>MPQSKSRKIAILGYRSVGKSSLTIQFVEGQFVDSNDPTIENTFTKLITVNGQEYHLQLVDTAGQDEYSIFPQTYSIDINGYILVYSVTSIKSFEVIKVIHGKLLDMVGKVQIPIMLVGNKKDLHMERVIS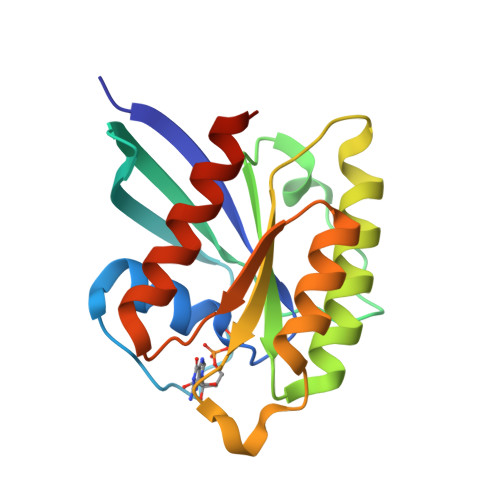YEEGKALAESWNAAFLESSAKENQTAVDVFRRIILEAEKLEHHHHHH[4x]>MSATLPDMDTLRERLLAGDRAALARAITLAESRRADHRAAVRDLIDAVLPQTGRAIRVGITGVPGVGKSTTIDALGSLLTAAGHKVAVLAVDPSSTRTGGSILGDKTRMARLAIDRNAFIRPSPSSGTLGGVAAKTRETMLLCEAAGFDVILVETVGVGQSETAVADLTDFFLVLMLPGAGDELQGIKKGIFELADMIAVNKADDGDGERRASAAASEYRAALHILTPPSATWTPPVVTISGLHGKGLDSLWSRIEDHRSKLTATGEIAGKRREQDVKWMWALVHERLHQRLVGSAEVRQATA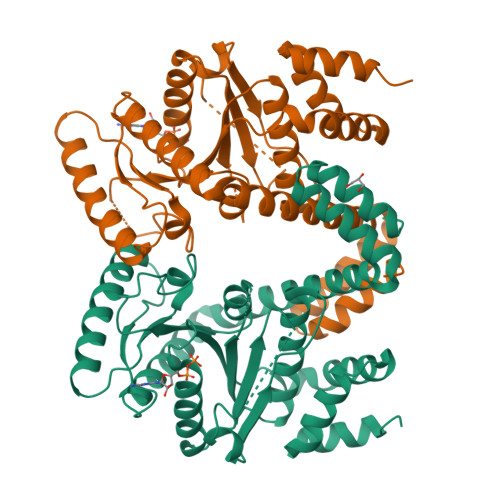EAERAVAGGEHSPAAGADAIATLIGLLEHHHHHH[2x]> MTNVLIEDLKWRGLIYQQTDEQGIEDLLNKEQVTLYCGADPTADSLHIGHLLPFLTLRRFQEHGHRPIVLIGGGTGMIGDPSGKSEERVLQTEEQVDKNIEGISKQMHNIFEFGTDHGAVLVNNRDWLGQISLISFLRDYGKHVGVNYMLGKDSIQSRLEHGISYTEFTYTILQAIDFGHLNRELNCKIQVGG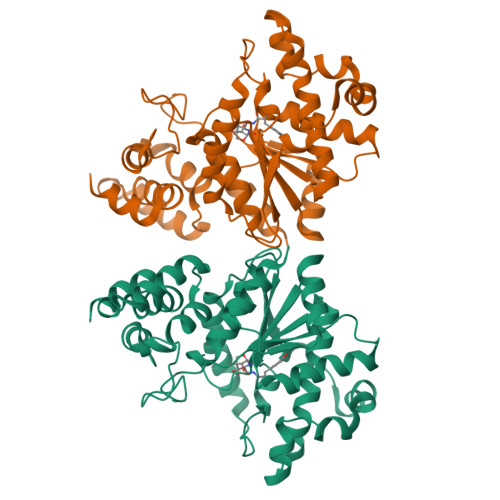SDQWGNITSGIELMRRMYGQTDAYGLTIPLVTKSDGKKFGKSESGAVWLDAEKTSPYEFYQFWINQSDEDVIKFLKYFTFLGKEEIDRLEQSKNEAPHLREAQKTLAEEVTKFIHGEDALNDAIRISQALFSGDLKSLSAKELKDGFKDVPQVTLSNDTTNIVEVLIETGISPSKRQAREDVNNGAIYINGERQQDVNYALAPEDKIDGEFTIIRRGKKKYFMVNYQ> MYCYYLHTSPASNENDVCHSASAKSNFIFPSFSSLVGFIVFFLWKRQMPLFHRLFVSGADLRGCHTALSSTFTQRRYWAKPKKRPKVGQGFHEKAQKWRDEFLLDRHRILADSLRAYVEFSASKRTE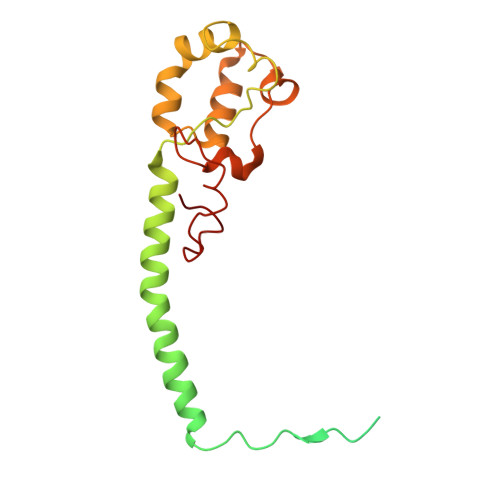PWDTRFRPFDRVEKDGVYVLMRHLMEDKFQLCNYHHRPVKRLFCNVGLLGPQVTTKARWKPYRYATNPANTSKAERIFQKDKTLYTHGHND>[2x]SMTEVKIKRLYTGDADFASQLDRLLAWSESEDTDIHQRVTEIIGCIRRDGDAALVELTARFDHFVVDTAAALELPRDVLEAAWQALPAEQAKALREAAERIRAYAERQKLDSWDYREADGTLLGQKITPLDRVGLYVPGGKAAYPSSVLMNAVPAKVAGVPELIMAVPAPRGELNA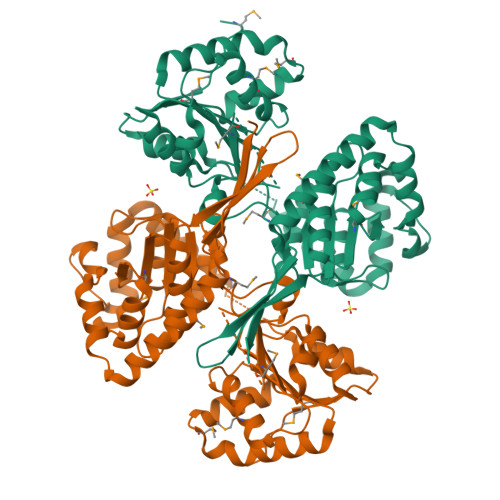LVLAAAYISGVDRVFRIGGAQAVAALAYGTETVPRVDKIVGPGNIYVATAKKLVFGQVGIDMVAGPSEILVISDGRTDPDWIAMDLFSQAEHDEDAQAILISPDAAHLEAVQASIERLLPGMERAEVIRTSLERRGGMILVDDLEQAAAVANRIAPEHLELSVESPEVLVESIRNAGAIFMGRYTAEALGDYCAGPNHVLPTSGTARFSSPLGVYDFQKRSSLIYCSPDGADQLGRTASLLAWGEGL>SKTIVLSVGEATRTLTEIQSTADRQIFEEKVGPLVGRLRLTASLRQNGAKTAYRVNLKLDQADVVDCSTSVCGELPKVRYTQVWSHDVTIVANSTEASRKSLYDLTKSLVATSQVEDLVVNLVPLGRAYGGSKTIVLSVGEATRTLTEIQSTADRQIFEEKVGPLVGRLRLTASLRQNGAKTAYRVNLKLDQADVVDCSTSVCGELPKVRYTQVWSHDVTIVAN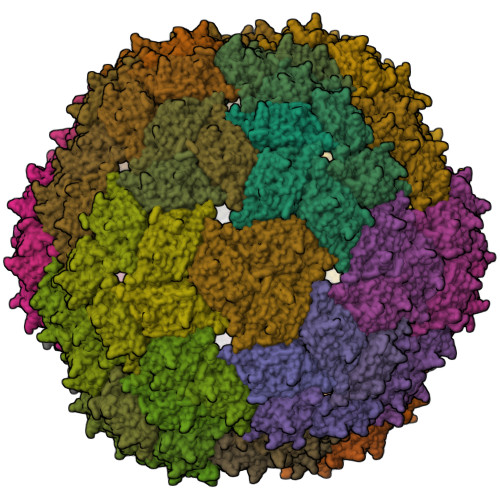STEASRKSLYDLTKSLVATSQVEDLVVNLVPLGR[120x]>[4x]MKYILVTGGVISGIGKGIIASSVGTILKSCGLHVTSIKIDPYINIDAGTFSPYEHGEVFVLDDGGEVDLDLGNYERFLDIRLTKDNNLTTGKIYQYVINKERKGDYLGKTV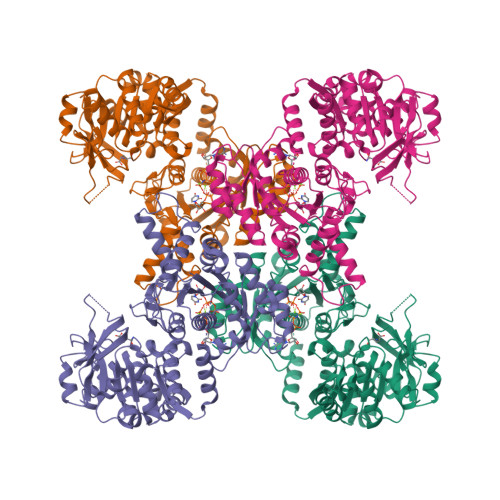QVVPHITDAIQEWVMRQALIPVDEDGLEPQVCVIELGGTVGDIESMPFIEAFRQFQFKVKRENFCNIHVSLVPQPSSTGEQKTKPTQNSVRELRGLGLSPDLVVCRCSNPLDTSVKEKISMFCHVEPEQVICVHDVSSIYRVPLLLEEQGVVDYFLRRLDLPIERQPRKMLMKWKEMADRYDRLLETCSIALVGKYTKFSDSYASVIKALEHSALAINHKLEIKYIDSADLEPITSQEEPVRYHEAWQKLCSAHGVLVPGGFGVRGTEGKIQAIAWARNQKKPFLGVCLGMQLAVVEFSRNVLGWQDANSTEFDPTTSHPVVVDMPEHNPGQMGGTMRLGKRRTLFQTKNSVMRKLYGDADYLEERHRHRFEVNPVWKKCLEEQGLKFVGQDVEGERMEIVELEDHPFFVGVQYHPEFLSRPIKPSPPYFGLLLASVGRLSHYLQKGCRLSPRDTYSDRSGSSSPDSEITELKFPSINHD> ANPLYQKHIISINDLSRDDLNLVLATAAKLKANPQPELLKHKVIASCFFEASTRTRLSFETSMHRLGASVVGFSDSANTSLGKKGETLADTISVISTYVDAIVMRHPQEGAARLATEFSGNVPVLNAGDGSNQHPTQTLLDLFTIQETQGRLDNLHVAMVGDLKYGRTVHSLTQALAKFDGNRFYFIAPDALAMPQYILDMLDEKGIAWSLHSSIEEVMAEVDILYMTRVQKERLDPSEYANVNAQ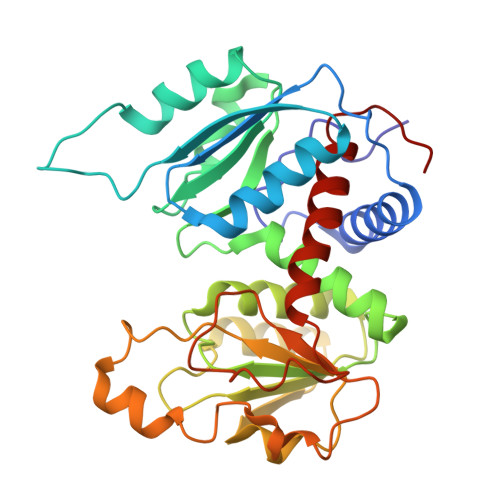FVLRASDLHNAKANMKVLHPLPRVDEIATDVDKTPHAWYFQQAGNGIFARQALLALVLNRDLVL>LMLHKRNICPIKGCGKNFFSHKYLVQHQRVHSDDRPLKCPWKGCKMTFKWAWSRTEHIRVHTGARPYVCAEPDCGQTFRFVSDFSRHKRKTG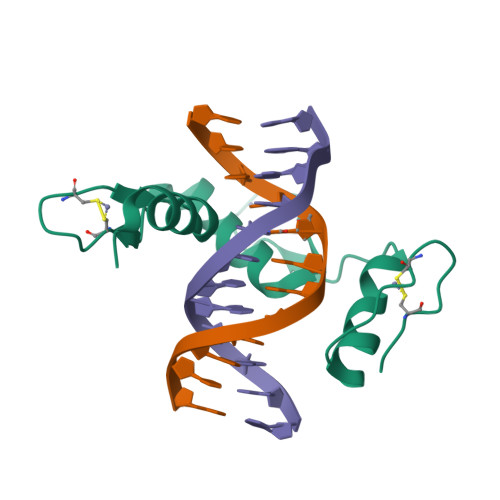HSVKKTNKR[2x]> MLRSTHPPPSSPSSSSSGGGGGGGSSASSSSEKTMVGGGGGGGGGSGSAAPSGAKLLQILNVRVVGSGERVVVLSHGFGTDQSAWSRVLPYLTRDHRVVLYDLVCAGSVNPDHFDFRRYDNLDAYVDDLLAILDALRIPRCAFVGHSVSAMIG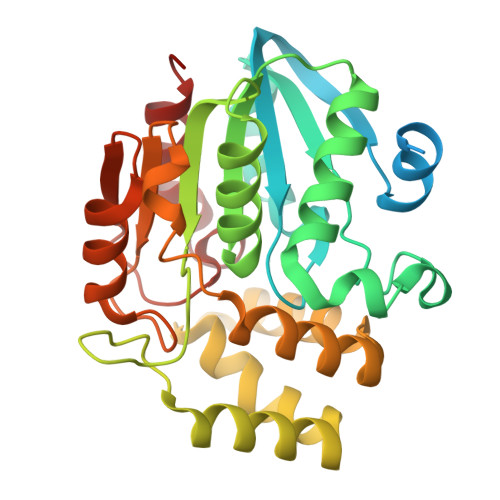ILASIRRPDLFAKLVLIGASPRFLNDSDYHGGFELEEIQQVFDAMGANYSAWATGYAPLAVGADVPAAVQEFSRTLFNMRPDISLHVCQTVFKTDLRGVLGMVRAPCVVVQTTRDVSVPASVAAYLKAHLGGRTTVEFLQTEGHLPHLSAPSLLAQVLRRALARY2-[(2~{R},5~{S})-2,5-dimethylmorpholin-4-yl]-~{N}-ethyl-ethanamide 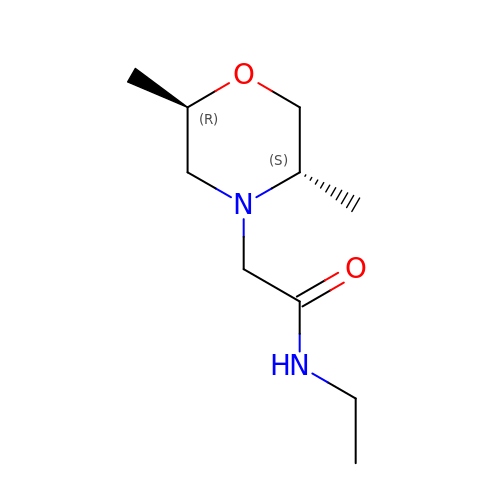| C10 H20 N2 O2 | YXUGPUQOOJOCPJ-DTWKUNHWSA-N> MHHHHHHKDEVALLAAVTLLGVLLQAYFSLQVISARRAFRVEPPLTTGPPEFERVYRAQVNCSEYFPLFLATLWVAGIFFHEGAAALCGLVYLFARLRYFQGYARSAQLRLAPLYASA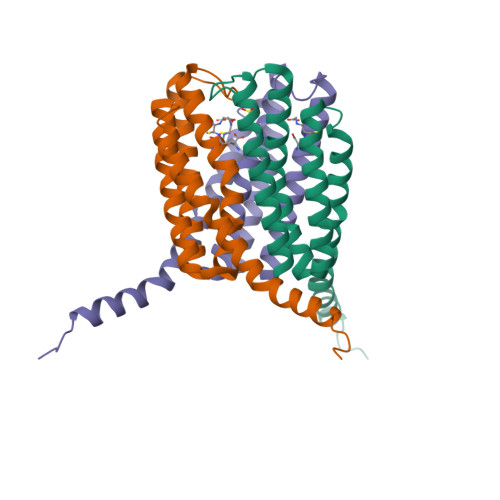RALWLLVALAALGLLAHFLPAALRAALLGRLRTLLPWA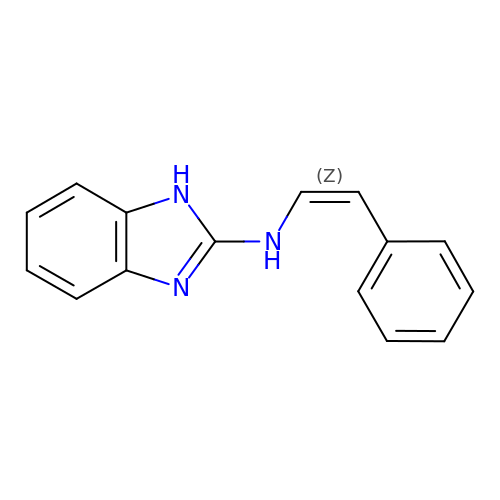N-[(Z)-2-phenylethenyl]-1H-benzimidazol-2-amine | C15 H13 N3 | NDQBJQDKEBGGFW-KHPPLWFESA-N> VVGGRVAQPNSWPWQISLQYKSGSSYYHTCGGSLIRQGWVMTAAHCVDSARTWRVVLGEHNLNTNEGKEQIM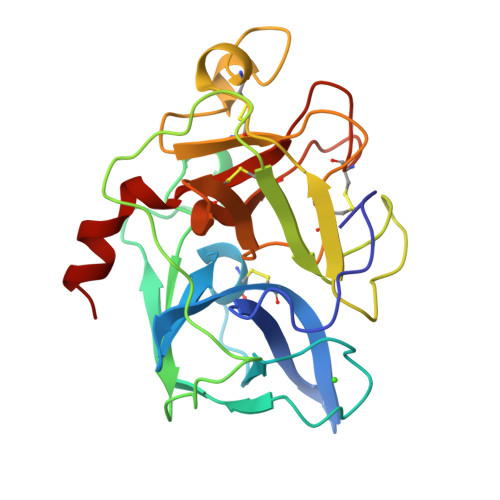TVNSVFIHSGWNSDDVAGGYDIALLRLNTQASLNSAVQLAALPPSNQILPNNNPCYITGWGKTSTGGPLSDSLKQAWLPSVDHATCSSSGWWGSTVKTTMVCAGGGANSGCNGDSGGPLNCQVNGSYYVHGVTSFVSSSGCNASKKPTVFTRVSAYISWMNGIM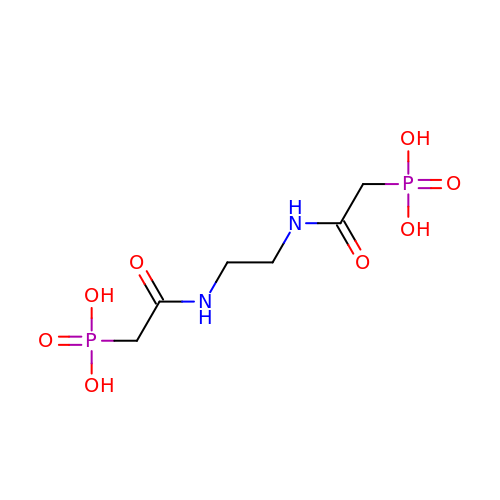{ETHANE-1,2-DIYLBIS[IMINO(2-OXOETHANE-2,1-DIYL)]}BIS(PHOSPHONIC ACID) | C6 H14 N2 O8 P2 | RPUNQQORCLHWTD-UHFFFAOYSA-N> MSVFDRLAGFADSVTNAKQVDVSTATAQKKAEQGVTTPLVSPDAAYQMQAARTGNVGANAFEPGTVQSDFMNLTPMQIMNKYGVEQGLQLINARADAGNQVFNDSVTTRTPGEELGDIATGVGLGFVNTLGGIGALGAGLLNDDAGAVVAQQLSKFNDAVHATQSQALQDKRKLFAARNLMNEVESERQYQTDKKEGTNDIVASLSKFGRDFVGSIENAAQTDSIISDGLAEGVGSLLGAGPVLRGASLLGKAVVPANTLRSAALAGAIDAGTGTQSLARIASTVGRAAPGMVGVGAMEAGGAYQQTADEIMKMSLKDLEKSPVYQQHIKDGMSPEQARRQTASETGLTAAAIQLPIAAATGPLVSRFEMAPFRAGSL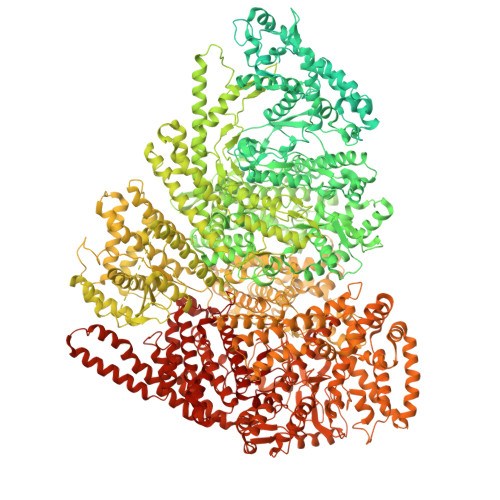GAVGMNLARETVEEGVQGATGQLAQNIAQQQNIDKNQDLLKGVGTQAGLGALYGFGSAGVVQAPAGAARLAGAATAPVLRTTMAGVKAAGSVAGKVVSPIKNTLVARGERVMKQNEEASPVADDYVAQAAQEAMAQAPEAEVTIRDAVEATDATPEQKVAAHQYVSDLMNATRFNPENYQEAPEHIRNAVAGSTDQVQVIQKLADLVNTLDESNPQALMEAASYMYDAVSEFEQFINRDPAALDSIPKDSPAIELLNRYTNLTANIQNTPKVIGALNVINRMINESAQNGSLNVTEESSPQEMQNVALAAEVAPEKLNPESVNVVLKHAADGRIKLNNRQIAALQNAAAILKGAREYDAEAARLGLRPQDIVSKQIKTDESRTQEGQYSALQHANRIRSAYNSGNFELASAYLNDFMQFAQHMQNKVGALNEHLVTGNADKNKSVHYQALTADREWVRSRTGLGVNPYDTKSVKFAQQVALEAKTVADIANALASAYPELKVSHIKVTPLDSRLNAPAAEVVKAFRQGNRDVASSQPKADSVNQVKETPVTKQEPVTSTVQTKTPVSESVKTEPTTKESSPQAIKEPVNQSEKQDVNLTNEDNIKQPTESVKETETSTKESTVTEELKEGIDAVYPSLVGTADSKAEGIKNYFKLSFTLPEEQKSRTVGSEAPLKDVAQALSSRARYELFTEKETANPAFNGEVIKRYKELMEHGEGIADILRSRLAKFLNTKDVGKRFAQGTEANRWVGGKLLNIVEQDGDTFKYNEQLLQTAVLAGLQWRLTATSNTAIKDAKDVAAITGIDQALLPEGLVEQFDTGMTLTEAVSSLAQKIESYWGLSRNPNAPLGYTKGIPTAMAAEILAAFVESTDVVENIVDMSEIDPDNKKTIGLYTITELDSFDPINSFPTAIEEAVLVNPTEKMFFGDDIPPVANTQLRNPAVRNTPEQKAALKAEQATEFYVHTPMVQFYETLGKDRILELMGAGTLNKELLNDNHAKSLEGKNRSVEDSYNQLFSVIEQVRAQSEDISTVPIHYAYNMTRVGRMQMLGKYNPQSAKLVREAILPTKATLDLSNQNNEDFSAFQLGLAQALDIKVHTMTREVMSDELTKLLEGNLKPAIDMMVEFNTTGSLPENAVDVLNTALGDRKSFVALMALMEYSRYLVAEDKSAFVTPLYVEADGVTNGPINAMMLMTGGLFTPDWIRNIAKGGLFIGSPNKTMNEHRSTADNNDLYQASTNALMESLGKLRSNYASNMPIQSQIDSLLSLMDLFLPDINLGENGALELKRGIAKNPLTITIYGSGARGIAGKLVSSVTDAIYERMSDVLKARAKDPNISAAMAMFGKQAASEAHAEELLARFLKDMETLTSTVPVKRKGVLELQSTGTGAKGKINPKTYTIKGEQLKALQENMLHFFVEPLRNGITQTVGESLVYSTEQLQKATQIQSVVLEDMFKQRVQEKLAEKAKDPTWKKGDFLTQKELNDIQASLNNLAPMIETGSQTFYIAGSENAEVANQVLATNLDDRMRVPMSIYAPAQAGVAGIPFMTIGTGDGMMMQTLSTMKGAPKNTLKIFDGMNIGLNDITDASRKANEAVYTSWQGNPIKNVYESYAKFMKNVDFSKLSPEALEAIGKSALEYDQRENATVDDIANAASLIERNLRNIALGVDIRHKVLDKVNLSIDQMAAVGAPYQNNGKIDLSNMTPEQQADELNKLFREELEARKQKVAKARAEVKEETVSEKEPVNPDFGMVGREHKASGVRILSATAIRNLAKISNLPSTQAATLAEIQKSLAAKDYKIIYGTPTQVAEYARQKNVTELTSQEMEEAQAGNIYGWTNFDDKTIYLVSPSMETLIHELVHASTFEEVYSFYQGNEVSPTSKQAIENLEGLMEQFRSLDISKDSPEMREAYADAIATIEGHLSNGFVDPAISKAAALNEFMAWGLANRALAAKQKRTSSLVQMVKDVYQAIKKLIWGRKQAPALGEDMFSNLLFNSAILMRSQPTTQAVAKDGTLFHSKAYGNNERLSQLNQTFDKLVTDYLRTDPVTEVERRGNVANALMSATRLVRDVQSHGFNMTAQEQSVFQMVTAALATEAAIDPHAMARAQELYTHVMKHLTVEHFMADPDSTNPADRYYAQQKYDTISGANLVEVDAKGRTSLLPTFLGLAMVNEELRSIIKEMPVPKADKKLGNDIDTLLTNAGTQVMESLNRRMAGDQKATNVQDSIDALSETIMAAALKRESFYDAVATPTGNFIDRANQYVTDSIERLSETVIEKADKVIANPSNIAAKGVAHLAKLTAAIASEKQGEIVAQGVMTAMNQGKVWQPFHDLVNDIVGRTKTNANVYDLIKLVKSQISQDRQQFREHLPTVIAGKFSRKLTDTEWSAMHTGLGKTDLAVLRETMSMAEIRDLLSSSKKVKDEISTLEKEIQNQAGRNWNLVQKKSKQLAQYMIMGEVGNNLLRNAHAISRLLGERITNGPVADVAAIDKLITLYSLELMNKSDRDLLSELAQSEVEGMEFSIAYMVGQRTEEMRKAKGDNRTLLNHFKGYIPVENQQGVNLIIADDKEFAKLNSQSFTRIGTYQGSTGFRTGSKGYYFSPVAARAPYSQGILQNVRNTAGGVDIGTGFTLGTMVAGRITDKPTVERITKALAKGERGREPLMPIYNSKGQVVAYEQSVDPNMLKHLNQDNHFAKMVGVWRGRQVEEAKAQRFNDILIEQLHAMYEKDIKDSSANKSQYVNLLGKIDDPVLADAINLMNIETRHKAEELFGKDELWVRRDMLNDALGYRAASIGDVWTGNSRWSPSTLDTVKKMFLGAFGNKAYHVVMNAENTIQNLVKDAKTVIVVKAVVVPAVNFLANIYQMIGRGVPVKDIAVNIPRKTSEINQYIKSRLRQIDAEAELRAAEGNPNLVRKLKTEIQSITDSHRRMSIWPLIEAGEFSSIADAGISRDDLLVAEGKIHEYMEKLANKLPEKVRNAGRYALIAKDTALFQGIQKTVEYSDFIAKAIIYDDLVKRKKKSSSEALGQVTEEFINYDRLPGRFRGYMESMGLMWFYNFKIRSIKVAMSMIRNNPVHSLIATVVPAPTMFGNVGLPIQDNMLTMLAEGRLDYSLGFGQGLRAPTLNPWFNLTH> MSSDASTYRLEDVLSSFYRVEKIKKINYHQYISKAQNDQWSIQMEFMLRKQDPKTLVALLSRDLWCFSINDDPVPTPPAIEHKPVSPDKIGTFTADYSKPNLPPHYALFLKALRRKIYINLALGSHNKLIQFGNACISLSGVPNYLVQLEPHLFVNGDLTVSLCAKNMGLVPMKEENLEESFLSKHALYLAPSGIRMHLAPASKQGYLITPPKHTELLLTTLSVSHGINLQNKKNLKWVAVVPDLGHLNGHTPTIASYLTPLLEAKKLVWPLHLIFAQPVADIENSTSGDPSEFHCLQDALDAIDDFIQLKQTAAYRTPGSSGVLSSNIAGTNPLSSDGAYTEQFQHYK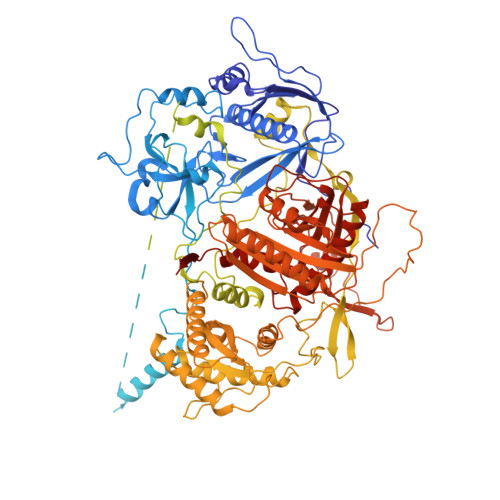NNSISSQPASYHSVQETNKISPKDFSPNFTGIDKLMLSPSDQFAPAFLNTPNNNINENELFNDRKQTTVSNDLENSPLKTELEANGRSLEKVNNSVSKTGSVDTLHNKEGTLEQREQNENLPSDKSDSMVDKELFGEDEDEDLFGDSNKSNSTNESNKSISDEITEDMFEMSDEEENNNNKSINKNNKEMHTDLGKDIPFFPSSEKPNIRTMSGTTKRLNGKRKYLDIPIDEMTLPTSPLYMDPGAPLPVETPRDRRKSVFAPLNFNPIIENNVDNKYKSGGKFSFSPLQKEEALNFDISMADLSSSEEEEDEEENGSSDEDLKSLNVRDDMKPSDNISTNTNIHEPQYINYSSIPSLQDSIIKQENFNSVNDANITSNKEGFNSIWKIPQNDIPQTESPLKTVDSSIQPIESNIKMTLEDNNVTSNPSEFTPNMVNSEISNLPKDKSGIPEFTPADPNLSFESSSSLPFLLRHMPLASIPDIFITPTPVVTISEKEQDILDLIAEQVVTDYNILGNLGIPKIAYRGVKDCQEGLITTTMLQLFSTFDRLNGNDTISKFYNMKQPYVFVKKHHELIKVKHDSQPFIKFLNFRPPNGIKNFKSLLLSSSFKEDCLSFAPTLSQTYINQELGFCELLKLTNEDPPGLMYLKAFDKNKLLLLAAQIVSYCSNNKNSIKNVPPILIILPLDNATLTELVDKANIFQVIKNEVCAKMPNIELYLKVIPMDFIRNVLVTVDQYVNVAISIYNMLPPKSVKFTHIAHTLPEKVNFRTMQQQQMQQQQQQQQQQQNNSTGSSSIIYYDSYIHLAYSRSVDKEWVFAALSDSYGQGSMTKTWYVGNSRGKFDDACNQIWNIALNLASKKFGKICLILTRLNGILPDDELMNWRRLSGRNIHLAVVCVDDNSKISFIDEDKLYPSFKPIYKDTRFGGRMDMTRLYDYEIRDIDQDIHGIVFQHPFPLAHSQHRCAIRSGALIKFKKCDGDTVWDKFAVNLLNCPHSDSTQLLETILEEFRNLAALNVWYGLSDGEDGHIPWHILAVKKMMNTLVHTRVKIANTSAATVHTATSSSIILSDK> YPRNPAMYSEEARLKSF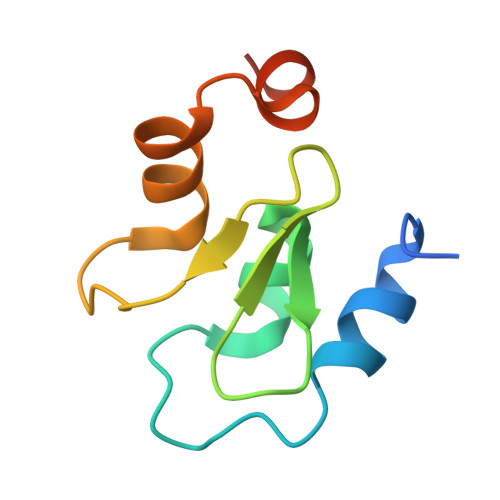QNWPDYAHLTPRELASAGLYYTGIGDQVQCFCCGGKLKNWEPCDRAWSEHRRHFPNCFFVLGRNLNIRSE>MFEARLVQGSILKKVLEALKDLINEACWDISSSGVNLQSMDSSHVSLVQLTLRSEGFDTYRCDRNLAMGVNLTSMSKILKCAGNEDIITLRAEDNADTLALVFEAPNQEKVSDYEMKLMDLDVEQLGIPEQEYSCVVKMPSGEFARICRDLSHIGDAVV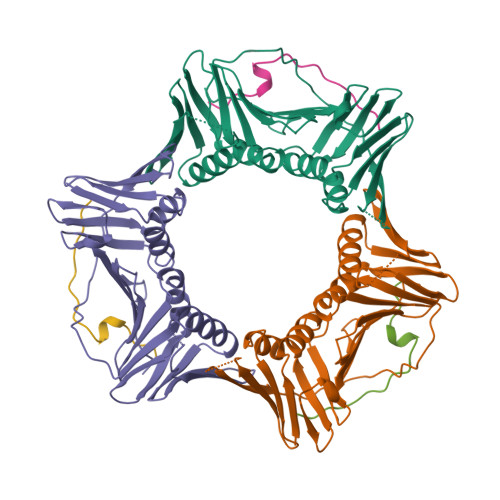ISCAKDGVKFSASGELGNGNIKLSQTSNVDKEEEAVTIEMNEPVQLTFALRYLNFFTKATPLSSTVTLSMSADVPLVVEYKIADMGHLKYYLAPKIEDEEGS[3x];>[3x]GRKRRQTSMTDFYHSKRRLIFS> MSLTDSKVKNAKSLEKEYKLTDGFGMHLLVHPNGSKYWRLSYRFEKKQRLLALGVYPAVSLADARQRRDEAKKLLAA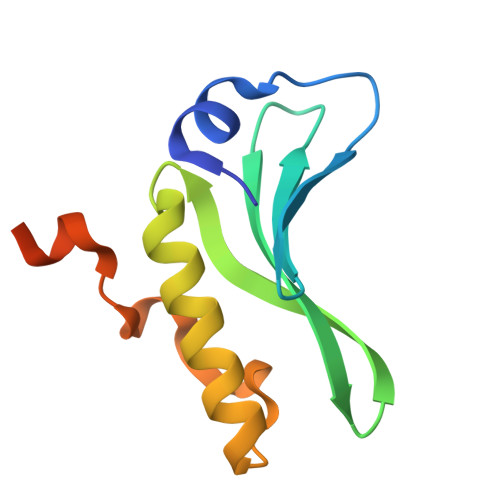GIDPSAKKQADNKTIQEKRNNTRLEHHHHHH> SLVQFET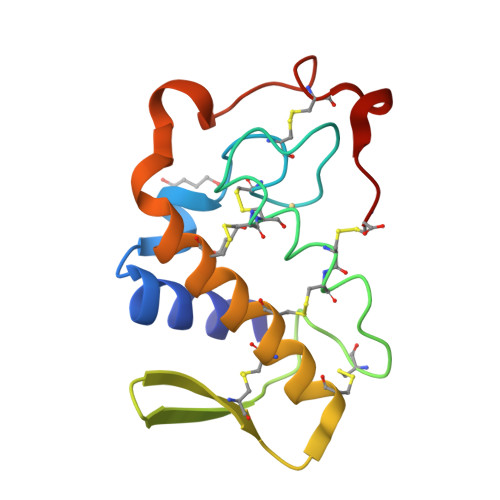LIMKVAKKSGMQWYSNYGCYCGWGGQGRPQDATDRCCFVHDCCYGKVTGCDPKMDVYSFSEENGDIVCGGDDPCKKEICECDRAAAICFRDNLNTYNDKKYWAFGAKNCPQEESEPC>[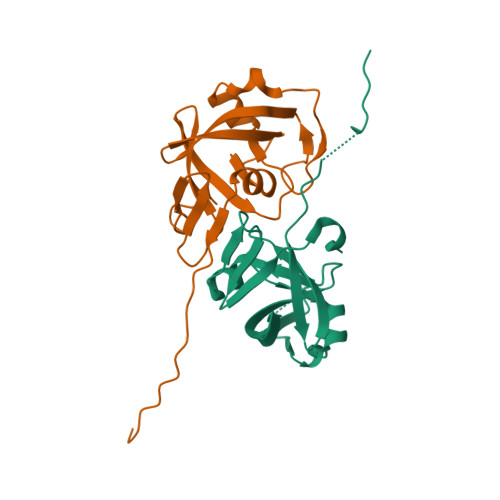2x]GPLGSEQLRNAIEYTPEMFTQVPMLYINIEINNYPVKAFVDTGAQTTIMSTRLAKKTGLSRMIDKRFIGEARGVGTGKIIGRIHQAQVKIETQYIPCSFTVLDTDIDVLIGLDMLKRHLACVDLKENVLRIAEVETSFLSEAEIPK>[2x]AKPDRSSFVPSLFSKKKKNVTMRSIKTTRDRVPTYQYNMNFEKLGKCIIINNKNFDKVTGMGVRNGTDKDAEALFKCFRSLGFDVIVYNDCSCAKMQDLLKKASEEDHTNAACFACILLSHGEENVIYGKDGVTPIKDLTAHFRGDRCKTLLEKPKLFFIQACRGTELDDGIQ;>ANPRYKIPVEADFLFAYSTVPGYYSWRSPGRGSWFVQALCSILEEHGKDLEIMQILTRVNDRVARHFESQ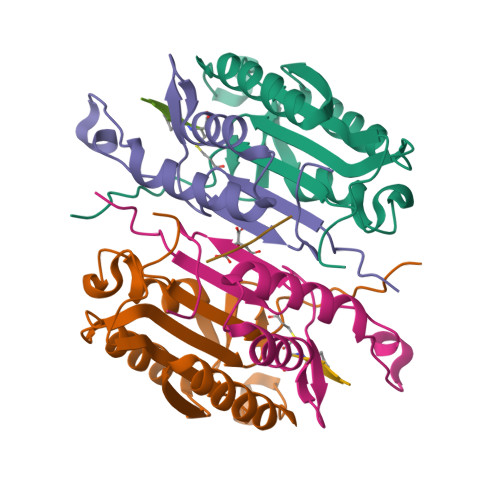SDDPHFHEKKQIPCVVSMLTKELYFSQ[2x];> QGHGE> GRI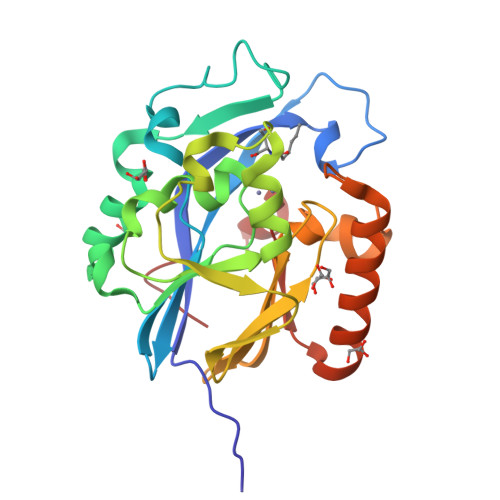SMTVKKLYFIPAGRCMLDHSSVNSALTPGKLLNLPVWCYLLETEEGPILVDTGMPESAVNNEGLFNGTFVEGQILPKMTEEDRIVNILKRVGYEPDDLLYIISSHLHFDHAGGNGAFTNTPIIVQRTEYEAALHREEYMKECILPHLNYKIIEGDYEVVPGVQLLYTPGHSPGHQSLFIETEQSGSVLLTIDASYTKENFEDEVPFAGFDPELALSSIKRLKEVVKKEKPIIFFGHDIEQEKSCRVFPEYI>MRIPLVGKDSIESKDIGFTLIHEHLRVFSEAVRQQWPHLYNEDEEFRNAVNEVKRAMQFGVKTIVDPTVMGIGRDIRFMEKVVKATGINLVAGTGIYIFIDLPFYFLNRSIDEIADLFIHDLKEGIQGTLNKAGFVKIAADEPGITKDVEKVIRAAAIANKETKVPIITHSNAHNNTGLEQQRILTEEGVDPGKILIGHLGDTDNIDYIKKIADKGSFIGLDRYGLDMSLPVDKRNETTLRLIKDGYSDKIMISHDYCCTIDLGTAKPEYKPKLAPRWSITLIFEDTIPFLKRNGVNEEVIATIFKENPKKFFS[4x]

Phosphotriesterase-like Lactonases (PLLs) are appealing candidates, being natural lactonases endowed with promiscuous phosphotriesterase activity. PTEs and PLLs belong to the amidohydrolase superfamily, and share the same (β/α)8 barrel topology. SsoPox exhibits high acyl-homoserine lactones and oxo-lactones hydrolysis abilities, and promiscuous, low phosphotriesterase activity. SsoPox is a very appealing candidate for the bioremediation of phosphotriesters because of its unique thermal stability, and its ability to resist aging, solvent and protease treatments.

Of them, the most active variants, αsA1 (C258L-I261F-W263A), αsA6 (F46L-C258A-W263M-I280T), αsB5 (V27A-I76T-Y97W-Y99F-L130P-L226V), αsC6 (L72I-Y99F-I122L-L228M-F229S-W263L), and αsD6 (V27A-Y97W-L228M-W263M) were subject to kinetic and structural characterization. Although the active sites of the improved variant structures superpose well onto the wt-structure, all selected mutants display altered loop 8 conformations. Changes are subtle for some of the variants (e.g. αsA1), but are large for others (e.g. αsC6). However, the active site cavities are larger for the mutants: most selected mutations replace residues with smaller ones: W263 is mutated into M/L/I, V27 into A, I76 into T, L130 into P, Y99 into F. Only two selected substitutions relate to bulkier side chains: Y97W and L228M. Interestingly, variants αsA6 and αsC6 exhibit enhanced lactonase activity against γ- and δ-lactones, while αsA1, αsB5 and αsD6 show reduced lactonase catalytic efficiencies.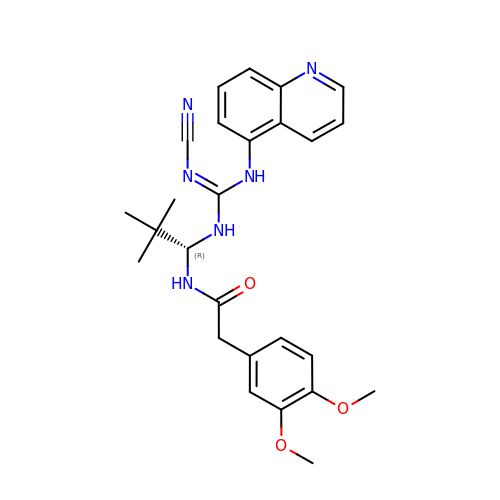N-{(1R)-1-[N''-cyano-N'-(quinolin-5-yl)carbamimidamido]-2,2-dimethylpropyl}-2-(3,4-dimethoxyphenyl)acetamide | C26 H30 N6 O3 | PUHSRMSFDASMAE-DEOSSOPVSA-N> MAHHHHHHVDDDDKMVHHDGFQTVKATIDWEHPMFKLYEKAKRNGKWNPADIDFSQDQKDFASLTSEEKISALPLVAGFSAGEEAVTLDILPMAHALARQGRLEDVLFLTTFMHDEAKHVEMFSRWQQAVGIGQMDLSVFHNDHYKRIFYEALPEAMNRLYADDSPEAVIRAATVYNMIVEGTLFESGYYTFRQIYKKAGLFPGLLQGIDYLNMDEGRHIQFGIYTIQRIVNEDERYYELFIRYMDELWPHVIGYVDYLTELGKRQQQLARTYALEIDYDL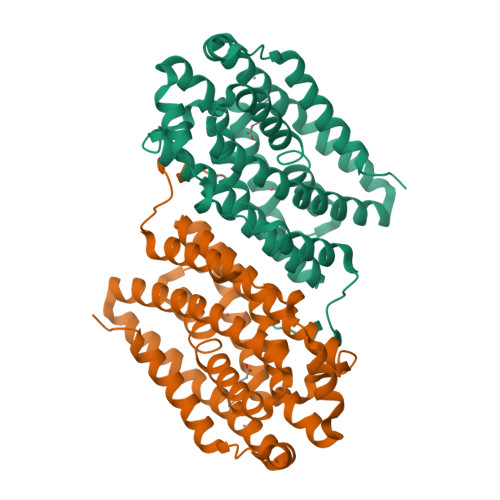LRHYVIKQFNLRKKQISRTKRVDVVEGLEKTAAES>[2x]MAMITGGELVVRTLIKAGVEHLFGLHGAHIDTIFQACLDHDVPIIDTRHEAAAGHAAEGYARAGAKLGVALVTAGGGFTNAVTPIANAWLDRTPVLFLTGSGALRDDETNTLQAGIDQVAMAAPITKWAHRVMATEHIPRLVMQAIRAALSAPRGPVLLDLPWDILMNQIDEDSVIIPDLVLSAHGARPDPADLDQALALLRKAERPVIVLGSEASRTARKTALSAFVAATGVPVFADYEGLSMLSGLPDAMRGGLVQNLYSFAKADAAPDLVLMLGARFGLNTGHGSGQLIPHSAQVIQVDPDACELGRLQGIALGIVADVGGTIEALAQATAQDAAWPDRGDWCAKVTDLAQERYASIAAKSSSEHALHPFHASQVIAKHVDAGVTVVADGALTYLWLSEVMSRVKPGGFLCHGYLGSMGVGFGTALGAQVADLEAGRRTILVTGDGSVGYSIGEFDTLVRKQLPLIVIIMNNQSWGATLHFQQLAVGPNRVTGTRLENGSYHGVAAAFGADGYHVDSVESFSAALAQALAHNRPACINVAVALDPIPPEELILIGMDPFA;>MAMITGGELVVRTLIKAGVEHLFGLHGAHIDTIFQACLDHDVPIIDTRHEAAAGHAAEGYARAGAKLGVALVTAGGGFTNAVTPIANAWLDRTPVLFLTGSGALRDDETNTLQAGIDQVAMAAPITKWAHRVMATEHIPRLVMQAIRAALSAPRGPVLLDLPWDILMNQIDEDSVIIPDLVLSAHGARPDPADLDQALALLRKAERPVIVLGSEASRT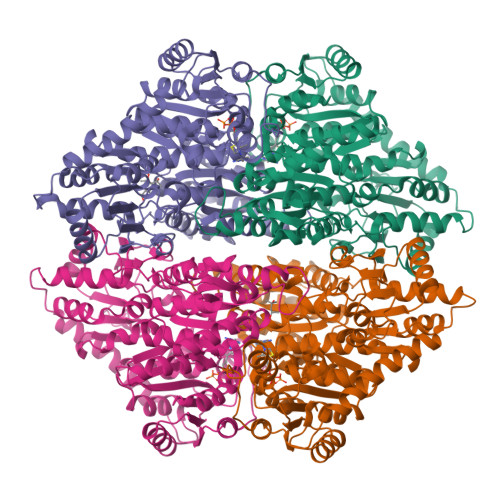ARKTALSAFVAATGVPVFADYEGLSMLSGLPDAMRGGLVQNLYSFAKADAAPDLVLMLGARFGLNTGHGSGQLIPHSAQVIQVDPDACELGRLQGIALGIVADVGGTIEALAQATAQDAAWPDRGDWCAKVTDLAQERYASIAAKSSSEHALHPFHASQVIAKHVDAGVTVVADGALTYLWLSEVMSRVKPGGFLCHGYLGSMGVGFGTALGAQVADLEAGRRTILVTGDGSVGYSIGEFDTLVRKQLPLIVIIMNNQSWGATLHFQQLAVGPNRVTGTRLENGSYHGVAAAFGADGYHVDSVESFSAALAQALAHNRPACINVAVALDPIPPEELIIIGMDPFA[2x]>[11x]MAALIAENFRFLSLFFKSKDVMIFNGLVALGTVGSQELFSVVAFHCPCSPARNYLYGLAAIGVPALVLFIIGIILNNHTWNLVAECQHRRTKNCSAAPTFLLLSSILGRAAVAPVTWSVISLLRGEAYVCALSEFVD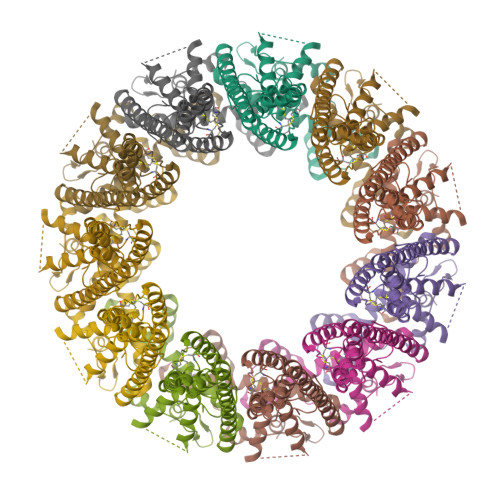PSSLTAREEHFPSAHATEILARFPCKENPDNLSDFREEVSRRLRYESQLFGWLLIGVVAILVFLTKCLKHYCSPLSYRQEAYWAQYRANEDQLFQRTAEVHSRVLAANNVRRFFGFVALNKDDEELIANFPVEGTQPRPQWNAITGVYLYRENQGLPLYSRLHKWAQGLAGNGAAPDNVEMALLPSGSAWSHPQFEK> MKAL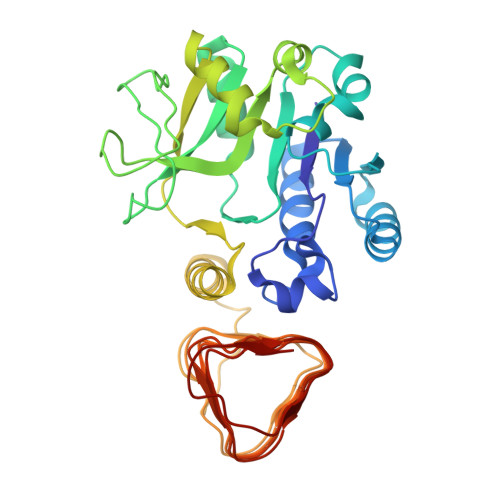ILVGGYGTRLRPLTLSTPKPLVDFCNKPILLHQVEALAAAGVDHVILAVSYMSQVLEKEMKAQEQRLGIRISMSHEEEPLGTAGPLALARDLLSETADPFFVLNSDVICDFPFQAMVQFHRHHGQEGSILVTKVEEPSKYGVVVCEADTGRIHRFVEKPQVFVSNKINAGMYILSPAVLQRIQLQPTSIEKEVFPIMAKEGQLYAMELQGFWMDIGQPKDFLTGMCLFLQSLRQKQPERLCSGPGIVGNVLVDPSARIGQNCSIGPNVSLGPGVVVEDGVCIRRCTVLRDARIRSHSWLESCIVGWRCRVGQWVRMENVTVLGEDVIVNDELYLNGASVLPHKSIGESVPEPRIIM>MNKVEPQESNAIRMIKEACEKNRRMMTDEAFRKEVEKRLYAGPSPELLAKLRVLWAANKEQ[4x];>[4x]MVKLSSDINLRDFGNNEYLSSVQDEAIRFATEQTDEILSLYSQHADTEGGRYVCADTFKELFPAFENKEDRATVNNAIHNSAAVLSSTQFDEVLKRDEPQKKEVIFVTGIPGSGATSTVKNMMMQDTTKLLFEGQLARPQSAFRKIEQCLERNLEVTIVAVSMRAERASDNTYKRFNEYGRGASIGIMADIQANLPDGLKQIRDKFGDAVKIVGINQDRNSEFIDKFDDVIKMLSL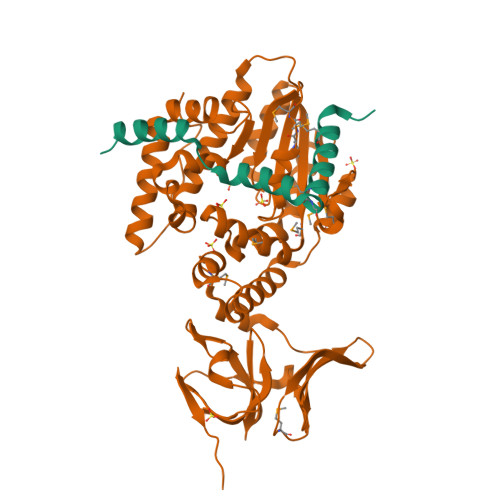GSQEQILGRLAEKIQSDFDSGKISRECFNQAKGSMDLESVFAKKEYSQQRVVTNSKGVTLETKSANELWSKVEQIPVTGMKAGIYLLGQAKKAETGQTYSGEIIYKDAAAVFQKTKNGLVRHNATHNEERLAKLVEIGQNVSIGSNKGKLIVKSLEYSAKKSISR> MYGKIIFVLLLSEIVSISASSTTGVAMHTSTSSSVTKSYISSQTNDTHKRDTYAATPRAHEVSEISVRTVYPPEEETGERVQLAHHFSEPEITLIIFGVMA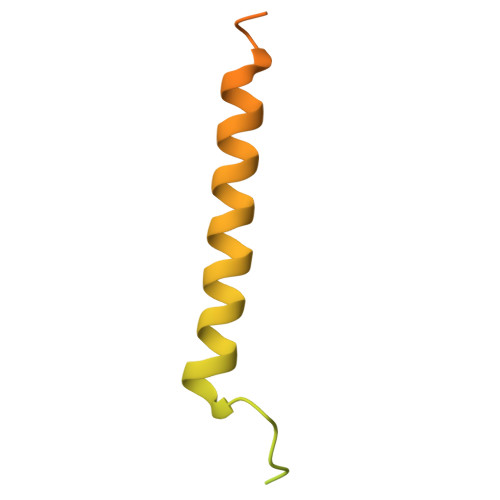GVIGTILLISYGIRRLIKKSPSDVKPLPSPDTDVPLSSVEIENPETSDQ>MYTNSDFVVIKALEDGVNVIGLTRGADTRFHHSEKLDKGEVLIAQFTEHTSAIKVRGKAYIQTRHGVIESEGKKAA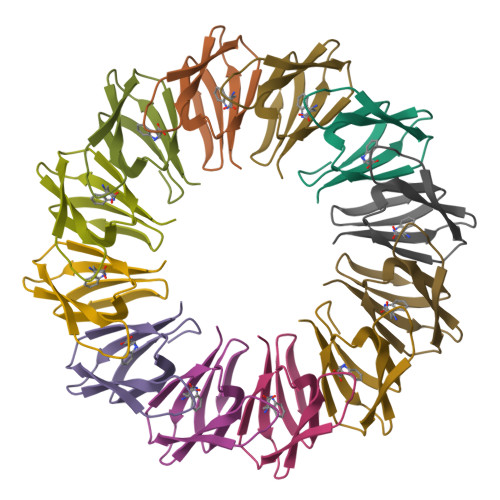AAA[3x]>KSCCPNTTGRDIYNTCRLGGGSRERCASLSGCKIISAST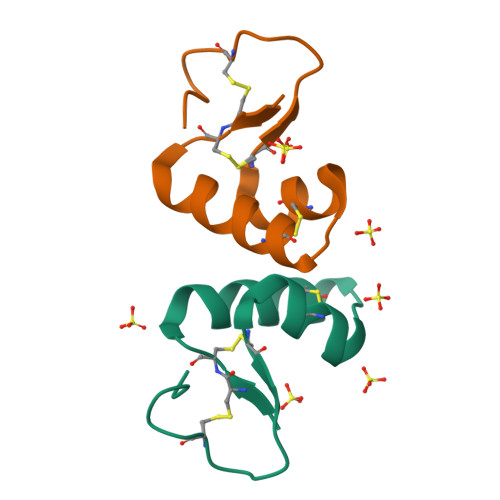CPSDYPK[2x]> VVHGQTAKTITIKVDTFKDRKPISPYIYGTNQDLAGDENMAARRLGGNRMTGYNWENNMSNAGSDWQHSSDNYLCSNGGLTQAECEKPGAVVTSFHDQSLKLGTYSLVTLPMAGYVAADGNGSVQESEAAPSARWNQVVNAKNAPFQLQPDLNDNYVYVDEFVHFLVNKYGTASTKAGVKGYALDNEPALWSHTHPRIHPEKVGAKELVDRSVSLSKAVKAIDAGAEVFGPVLYGFGAYKDLQTAPDWDS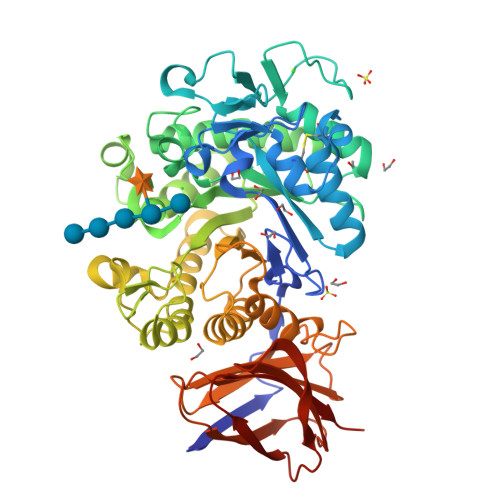VKGNYSWFVDYYLDQMRLSSQVEGKRLLDVFDVHWYPEAMGGGIRITNEVGNDETKKARMQAPRTLWDPTYKEDSWIAQWFSEFLPILPRLKQSVDKYYPGTKLAMTSYSYGGENDISGGIAMTDVLGILGKNDVYMANYWKLKDGVNNYVSAAYKLYRNYDGKNSTFGDTSVSAQTSDIVNSSVHASVTNASDKELHLVVMNKSMDSAFDAQFDLSGAKTYISGKVWGFDKNSSQIKEAAPITQISGNRFTYTVPPLTAYHIVLTTGNYTSPV>[4x]AEMGAAACTLLWGVSSSEEVVKAILGGDKALKFFSITGQTMES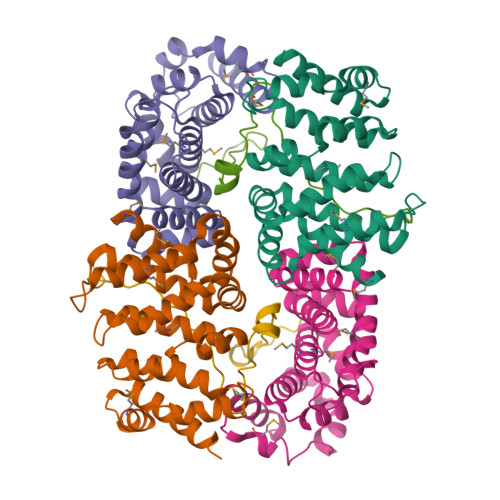FVKSLDGDVQELDSDESQFVFALAGIVTNVAAIACGREFLVNSSRVLLDTILQLLGDLKPGQCTKLKVLMLMSLYNVSINLKGLKYISESPGFIPLLWWLLSDPDAEVCLHVLRLVQSVVLEPEVFSKSASEFRSSLPLQRILAMSKSRNPRLQTAAQELLEDLRTLEHNV;>[2x]NEFDRIIENQEKSLKASKSTPDGTIKDRRLFMHHVSLEPITTVPFRTTKERQENLYFQG> MRIMAQRLKELQREIDKKKKERIAEAYLSSVEVTNSSPSLSKQDDALTLPKVSPFLDSTPFTTLHNSLYGQQIHSIDDELAQICKLEYELQTQIADEQITALKHFLTIRTGSPQEIQYVDKEWMKSNQHVPSFLGDVKLMFGDTAGKFRSTSKSVDSIHSITSDVQVTRKKQTRSQIRNSYRVQKKHKVQQPLKPNTLYVYKYKGLPRVVLRFVPKVDTTSNSNSSSASDSKKDKDAFSCDDLSPTWKYILTEAKRAFPDRSYSDCIHPMTWEEWLEENQDHVKVLTQYAHQLDYVTLLQDFNLYVSGGASRVRNIDMSTLPTSINVLDHFELYGDASMKEYVRSGEWYGLLREIEQEGMTVNESEKVFANPDTYVLNVKKYFLRRFQQEIASTGMTPLTDELLNIMFVHWNIIVTAEPKLQVIKDDLLKYYSRYGVDATFDYNMKRSEMTVVTRGHLLAHKVLECALRIVETIYTYDIQDETFKDILIDLGRLIMRDPIYGTTTVRDATTVMKQLMYTQGTQFRRIMFKKYDYSNFNEKLVLKGEQMTNEPPTLLATTHYEEMDKKRIDALIKANQRAGNILSQSSIERCRYTDSLDLVGDA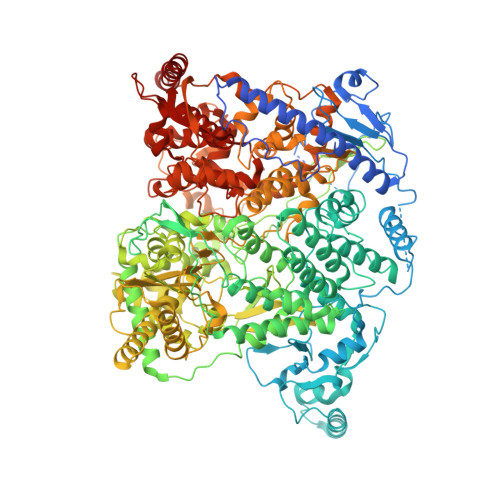NRYFSALTTLEAVAGFASSDLLSGFIDSNESIEFTGTAHLRKLLYHSVREQITTLNTSTVPRPSLPKVLLSSAKDTASASIEPLTFRIYKTTPEYDGESLNLVESTVEMSTRQKKPNLMKAAEILRSTVTTNQEMIISGGTRAVQGGKGARAVYPTKQPYHIAGSLLFHKVDTIVNANKKYRGVSNKYGQGISNAIPHIGVPEIIAVSSDGMAICLALDVSAFDVAQKYTEADIELAMRDGFLDSEISMISGETVLERMNPADLANNLLTNTPPRYKYQTALGDIIILQHDNRSGVPWTGTQNDLVNVSNHHMAYDEYKKRVAELQRQGKISIDVNDKHHIVRVFGDDSTFIMTYDEPPSAEEVHLMCATFVESYQDTAGTLGFAINARKGMIGRYGSEYLKNSAIYGNIKSVNQVKFRGSEKSASYHFGVSEKVSMIRDITDLTITRGCDETRKWKYNLMMLPVDLTTRAGAFRMHNLCSIMTGVGKMYLGGTLNNKLIASYHGSSFGWNFDDNLIKTANSIGAISDSSYDAISTKITNLADFKDSQQRITRDIITSGRLPQHLNRYGKSNILRHILASAAMGPLSQIEKNVNAYNVVMGILNGKLEAPTVLERLNMGFKYVVMSDLKQDDYSPYSCQGLQYRRMLVHWGLNDSRITSFDPKGKLQHLLAKNSQILPIHFDIEFVYRLYLQAGTMGFLQVMSYYQLPDTLTHEMLAAVVALELQLGNDKYAVDMGVYSSQAGQIRINDALMDSIIQHRRGPPLPIIDRTLNRLLLHTYMLMFGLMGKSIDSTKIDPTLSWRAILESNDQRIAQLSELLTAV>GSLAEVQALETLLARELSVFLTEPGSKKTNIINRITGKTYALPSTELLRFYEHLEQCRKQGALMYFLERQGTYSGLMLDYDLKLNTNAAPSLESSVLSRLCHRIFVHIKNSSVLPEGSHKIHFFFTLKPEAVQGKYGFHVLIPGLKMAASTKKSIIASLQHDATVQKILHEQGVANPESCLDPHSASVPSLLYGSSKLNHRPYQLKTGFELVFDSSDPDYIPIHQIKNIESYNLVSELSLTNEQGSLVRPVYCA[2x]

Here, we report the structural and biochemical studies of the highly conserved C962R protein of ASFV, showing that C962R is a multidomain protein. The N-terminal AEP domain is responsible for the DNA polymerization activity, whereas the DNA unwinding activity is catalyzed by the central SF3 helicase domain. The middle PriCT2 and D5_N domains and the C-terminal Tail domain all contribute to the DNA unwinding activity of C962R. C962R preferentially works on forked DNA, and likely functions in Base-excision repair (BER) or other repair pathway in ASFV.

Based on above structural observations, we constructed one new AEP variant (aa 21–272) and performed co-crystallization trials. One AEP-Mn2+ binary complex was solved at atomic resolution, revealed the detailed coordination of Mn2+ ions. The A-site Mn2+ coordinates with the side chains of Asp97 and Asp99 and three water molecules. Two of the water molecules form hydrogen bonding (H-bond) interactions with His157 or Tyr221, whereas the third water molecule coordinates with the B-site Mn2+. In addition to Asp97 and Asp99, the B-site Mn2+ also coordinates with the side chain of Asp200. Structural superposition showed that coordination of Mn2+ can dramatically change the conformation of Asp99 side chain. Structural comparison revealed that the orientations of the two Mn2+ ions are similar in the binary and ternary complex structures; the root mean square deviation (RMSD) values between the two complex structures and the apo-AEP structure are around 0.6–1.0 Å. The Leu21-Val37 region folds into one helix (α2) in the apo-form AEP structure, but it is disordered in the binary and ternary structures of the AEP domain.N-methyl-4-pyridin-4-yl-1H-pyrrole-2-carboxamide | C11 H11 N3 O | 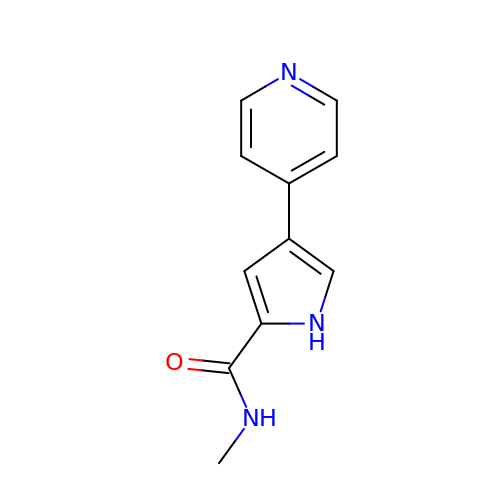CUQAMHMOOUOTLK-UHFFFAOYSA-N>[2x]QQVGTQTAENHPKLTVSQCSAGGSCTTESRSVVLDSNWRWLHTTSGTTNCYTGNTWDASLCPDPVT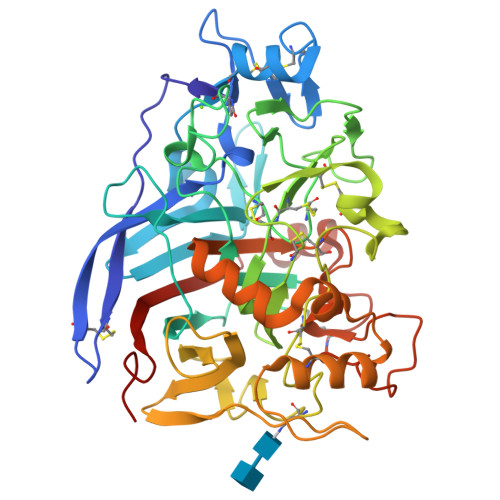CAQNCALDGADYSGTYGISTSGNALTLKFVTNGPYSTNIGSRVYLMSADDTNYEIFKLKNQEFAFDVDMSNLPCGLNGALYFVEMDADGGLSRFPNNKAGSKYGTGYCDTQCPQDIKFINGEANILGWTPSSSDSNAGTGQYGSCCNEMDVWEANINSAAVTPHVCNVQGQTRCSGTQCGDGDERYDGICDKDGCDFNSFRMGNQTFLGPGKTVNTNSKFTVVTQFLTSDNTTTGTLHEIRRLYVQNGKVIANSKTNIAGMSQFDSITDDFCNAQKTAFGDTNSFENLGGLNVMGQAFDKGVVLVMSVWDDHEANMLWLDSDYPTTSSASTPGVARGTCATTSGVPANVESQNPNSSVVFSNIKIGPIGSTYTA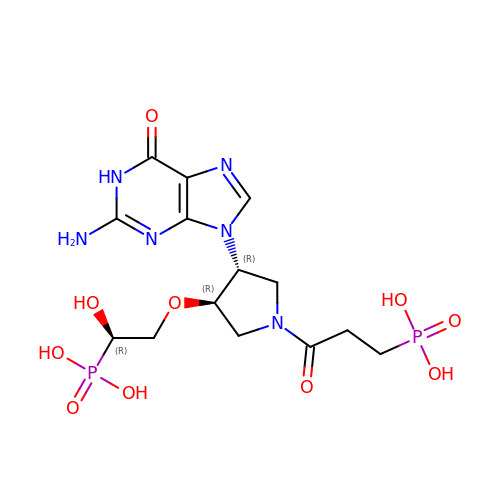(3-{(3R,4R)-3-(2-amino-6-oxo-1,6-dihydro-9H-purin-9-yl)-4-[(2R)-2-hydroxy-2-phosphonoethoxy]pyrrolidin-1-yl}-3-oxopropyl)phosphonic acid | C14 H22 N6 O10 P2 | RBYFDIJTTUISNF-NQMVMOMDSA-N octane-1,1-diol | C8 H18 O2 | 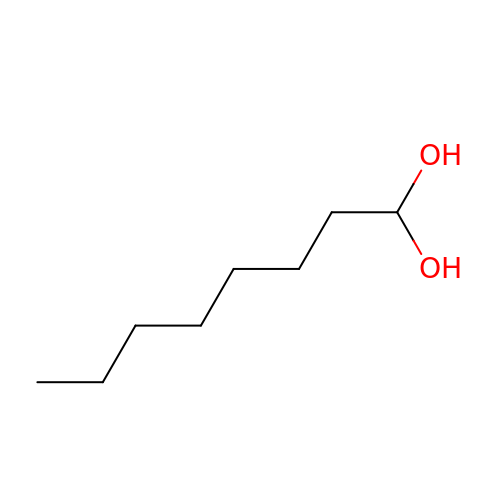QYPUTBKHHRIDGS-UHFFFAOYSA-N> MALTKAEMSEYLFDKLGLSKRDAKELVELFFEEIRRALENGEQVKLSGFGNFDLRDKNQRPG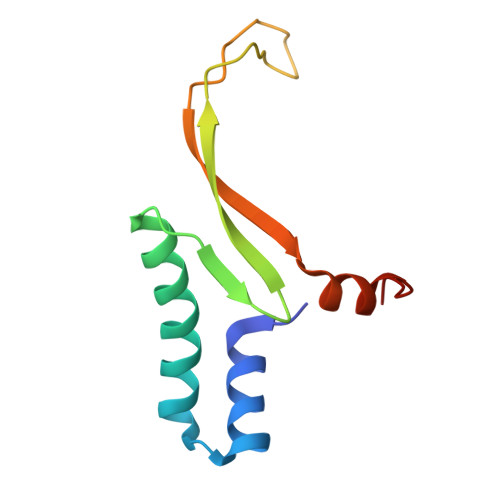RNPKTGEDIPITARRVVTFRPGQKLKSRVENASPKDE(3Beta,5alpha)-3-Hydroxyandrostan-17-one | C19 H30 O2 | 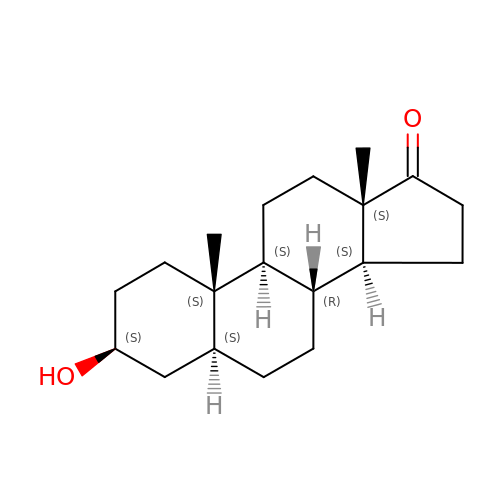QGXBDMJGAMFCBF-LUJOEAJASA-N>[4x]MDFLDRNAAPLNEGEWQRIDEAVVSTARRTLVARRIIDVLGPLGSGVYSIPYSVFSGKSPTGIDMVGENEEFVVEASRRATINLPILYKDFKIMWRDVEADRHLGLPIDVSTAAVAGNFVAVQEDHLIFNGNVELGHDGLFTVKDRQTVAISDWNETGAALADVVKAVGALSQAGHYGPYAMVVSPVLFGRMIRVFGWTGMLELDQVKALITG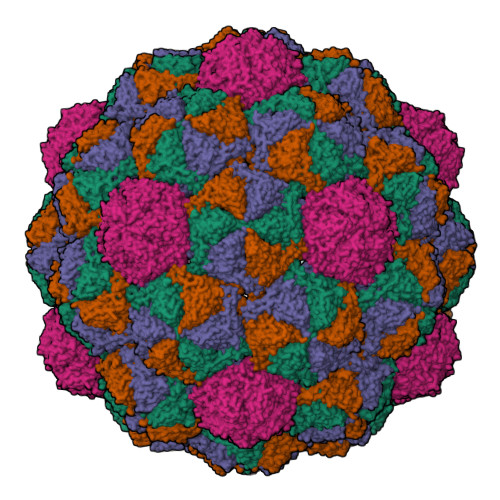GVHYSNVIGGSKAVVVATGSQNLNLALGQDMVTAYMGPTSMNHVFRVLETAALLVRRPDAICTIE> GIKRLRRLYCNVGIGFHLQALPDGRIGGAHADTRDSLLELSPVERGVVSIFGVASRFFVAMSSKGKLYGSPFFTDECTFKEILLPNNYNAYESYKYPGMFIALGKNGKTKKGNRVSP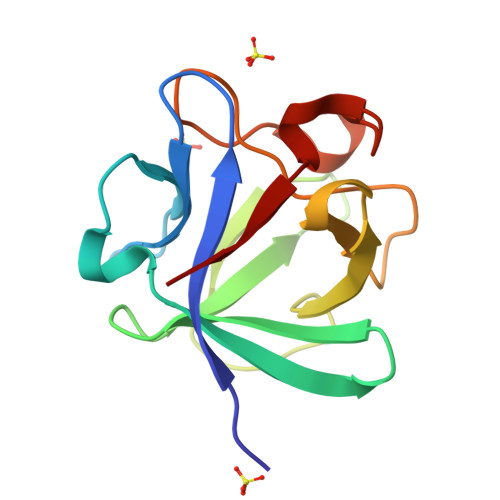TMKVTHFLPRL>[2x]GPLGSMANRDDIDASAVMAAYLAREYAEAVEEQLTPRERDALEALRVSGEEVRSPLLQELSNAGEHRANPENSHIPAALVSALLEAPTSPGRMVTAVELCAQMGRLWTRGRQLVD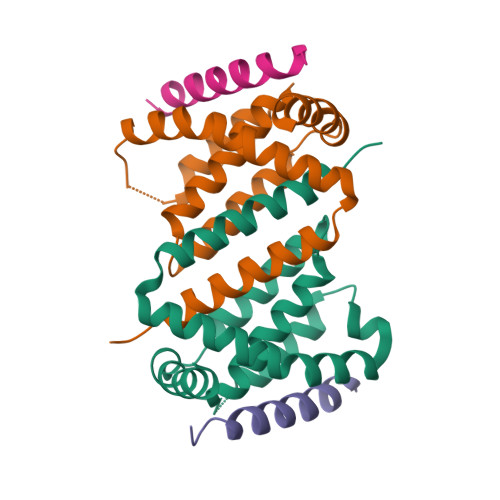FMRLVYVLLDRLPPTADEDLGAWLQAVARVHGT;>EEQWAREIGAQLRRMADDLNAQYERR[2x]>[2x]GSAKDPAASKSFAIQHSLANMEQMQKDIADSKNVLTQTENTLQGVLKSLTRADQLTVQALNGTNSEKELQAIGVEIDQILKQVVYLANTKEQGRYIFGGDSAENLPFTEDGTYQGGKNDVNWKLNDGYEFKAFRNGEALLSPVIKTLKQMSEAMQNGDQKALKPLLEENKQNLDGIINRTTEVGSTMNTMETFKTILSEQNVALQENRKEIED

To initiate filament growth, three junction proteins, namely, FlgK (hook-associated protein 1), FlgL (hook-associated protein 3), and the cap protein FliD (hook-associated protein 2), are sequentially placed at the distal end of the hook. The FlgL and FlgK junction proteins that are located between the FlgE hook and the flagellin filament are indispensable for the formation of the flagellum because both FlgL-deficient bacteria and FlgK-deficient bacteria lack functional flagella and are immotile. To investigate the role of FlgL in hook-filament assembly, we have determined the crystal structures of FlgL from gram-positive Bacillus cereus (bcFlgL) and gram-negative Xanthomonas campestris (xcFlgL). The bcFlgL and xcFlgL structures revealed that the D1 domain of FlgL forms a four-segment structure, irrespective of the bacterial species.

Crystal structures for the truncated bcFlgL and xcFlgL proteins (residues 45–251 and residues 48–364, respectively), which lack ~45 N-terminal residues and ~35 C-terminal residues, were solved by multiwavelength anomalous diffraction (MAD) phasing and single-wavelength anomalous diffraction (SAD) phasing, respectively. Although bcFlgL and xcFlgL are orthologous, they structurally differ in the number of domains. The truncated bcFlgL and xcFlgL proteins adopt one-domain (D1) and two-domain (D1-D2) structures, respectively. The D1 domains of bcFlgL and xcFlgL are superimposable, with the same organization of four α-helices (α1-α4) and one β-hairpin (β3-β4 hairpin), although the β1-β2 hairpin is located in different positions. Among the flagellar components, the D1 domain of FlgL exhibits the highest structural similarity to that of flagellin, with a root-mean-square deviation (RMSD) value of 1.90 Å between the D1 domains of bcFlgL and S. Typhimurium flagellin for 140 Cα atoms. The D1 domains of FlgL and flagellin both contain a three-α-helix bundle and a β-hairpin, with a similar length for each segment. The FlgL N-terminal portion that is missing in the bcFlgL structure is relatively short (44 residues), and the terminal regions of FlgL are highly likely to form α-helices based on secondary structure prediction, suggesting that the D0 domain of FlgL adopts a coiled-coil structure that consists of two α-helices, as observed for flagellin.> GPHMTDEDVKKWREERKKMWLL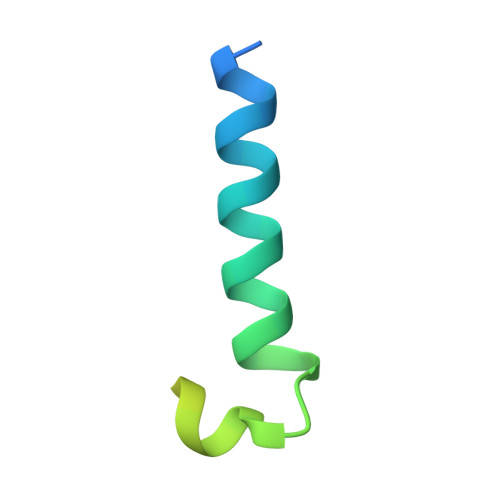KISNNKQKHMQEMGIKEDELKSQPSIFKESRKEKQ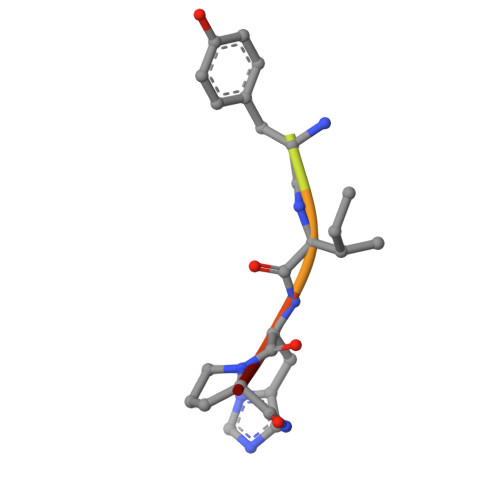> DRVYIHPF> GRGYEIPARLRTLHNLVIQYASQGRYEVAVPLCKQALEDLEKTSGHDHPDVATMLNILALVYRDQNKYKDAAHLLNDALAIREKTLGKDHPAVAATLNNLAVLYGKRGKYKEAEPLCKRALEIREKVLGKFHPDVAKQLSNLALLCQNQGKAEEVEYYYRRALEIYATRLGPDDPNVAKTKNNLASCYLKQGKYQDAETLYKEILTRAHEKEFGSVNGENKPIWMHAEEREESKDKRRDSAPYGEYGSWYKACKVDSPTVNTTLRS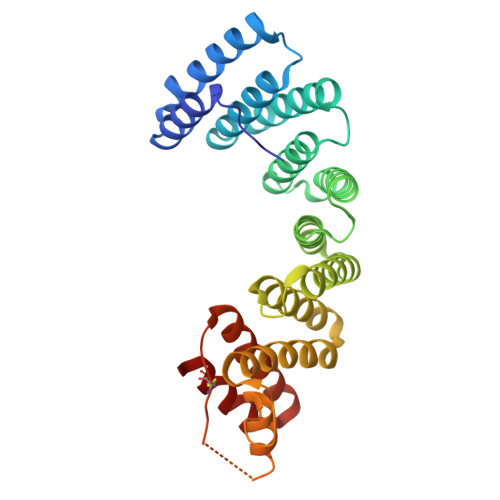LGALYRRQGKLEAAHTLEDCASRSR> LN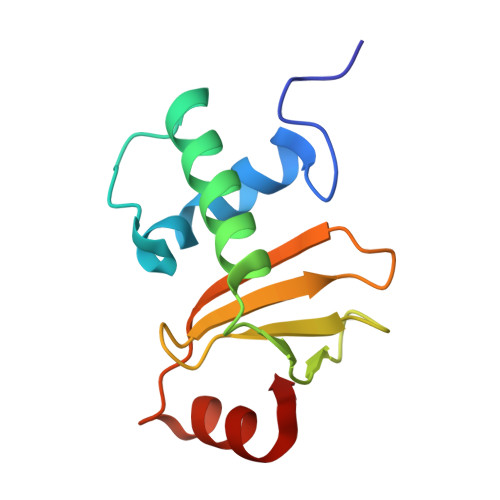DPLDSGRFSRKQLDKKYKHAGDFGISDTKKNRETLTKFRDAIEEHLSDKDTVEKGTYRREKGSKVYFNPNTMNVVIIKSNGEFLSGWKINPDADNGRIYLETGEL> MNLVLMGLPGAGKGTQGERIVEDYGTPHISTGDMFRAAMKEETPLGLEAKSYIDKGELVPDEVTIGIVKERLGKDDCERGFLLDGFPRTVAQAEALEEILEEYGKPIDYVINIEVDKDVLMERLTGRRICSVCGTTYHLVFNPPKTPGIC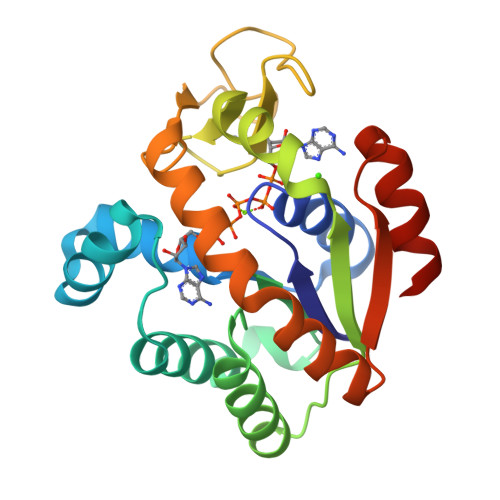DKDGGELYQRADDNEETVSKRLEVNMKQTQPLLDFYSEKGYLANVNGQQDIQDVYADVKDLLGGLKK>AAPPAPPVSYGVEEDVFHPVRAKQGMVASVDATATQVGVDILKEGGNAVDAAVAVGYALAVTHPQAGNLGGGGFMLIRSKNGNTTAIDFREM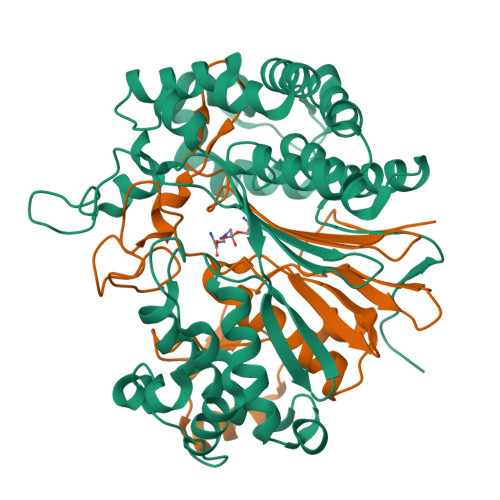APAKATRDMFLDDQGNPDSKKSLTSHLASGTPGTVAGFSLALDKYGTMPLNKVVQPAFKLARDGFIVNDALADDLKTYGSEVLPNHENSKAIFWKEGEPLKKGDTLVQANLAKSLEMIAENGPDEFYKGTIAEQIAQEMQKNGGLITKEDLAAYKAVERTPISGDYRGYQVYSMPPPSSGGIHIVQILNILENFDMKKYGFGSADAMQIMAEAEKYAYADRSEYLGDPDFVKVPWQALTNKAYAKSIADQIDINKAKPSSEIRPGKLAPYESNQ[2x];>TTHYSVVDKDGNAVAVTYTLNTTFGTGIVAGESGILLNNQMDDFSAKPGVPNVYGLVGGDANAVGPNKRPLSSMSPTIVVKDGKTWLVTGSPGGSRIITTVLQMVVNSIDYGLNVAEATNAPRFHHQWLPDELRVEKGFSPDTLKLLEAKGQKVALKEAMGSTQSIMVGPDGELYGASDPRSVDDLTAGY[2x]[(2~{R})-2-oxidanyl-3-[oxidanyl-[2-(trimethyl-$l^{5}-azanyl)ethoxy]phosphoryl]oxy-propyl] hexadecanoate 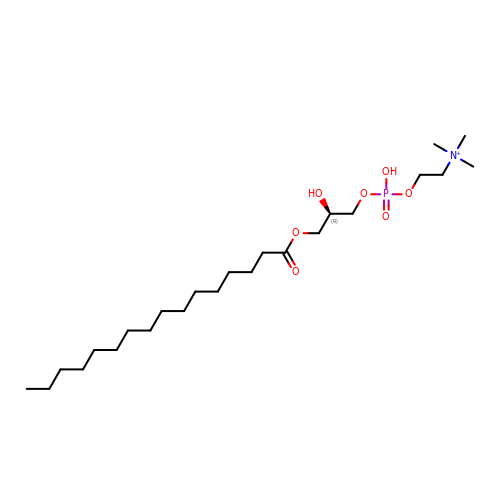| C24 H51 N O7 P | ASWBNKHCZGQVJV-HSZRJFAPSA-O>MAVFEQNKRPKISLIGSGMIGGTMAYLCALKELGDVVLFDVVKNMPQGKALDLSHSTSVADTNVKVTGTNSYEDIKGSDVVIITAGLTKVPGKSDKEWSRDDLLPINAKIMKEVGENIKKYCPNAFVICITNPLDVMVKVLQEASGLPHNKVCGMAGVLDSSRFRYFIAEK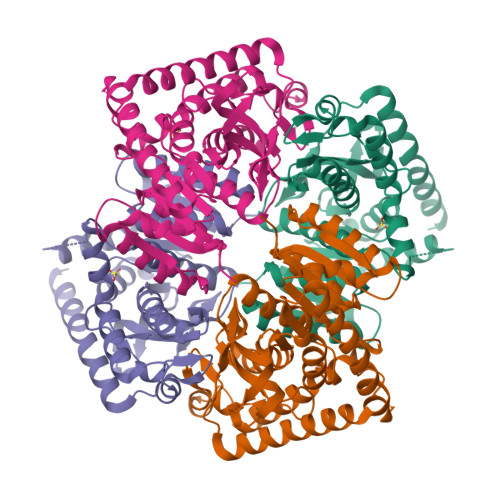LNVSPRDVQAMVIGAHGDNMVPLPRYVTVNGIPLQEFIKKGWITQEEIDEIVERTRNAGGEIVNLLGTGSAYFAPAASAIAMAEAYLKDQKRVLPCSCYLEGQYGVKDLYVGVPVVIGGNGVEKVIELELTPEEKEMFDKSIEEVRELVKALEALDAPA[2x]> MAPKATLVKKFKGLAVGVGALLAAPPIMGLASYAVNGISSYLSITINSTTYDFAPLAQAVMVFGGIGLVAYG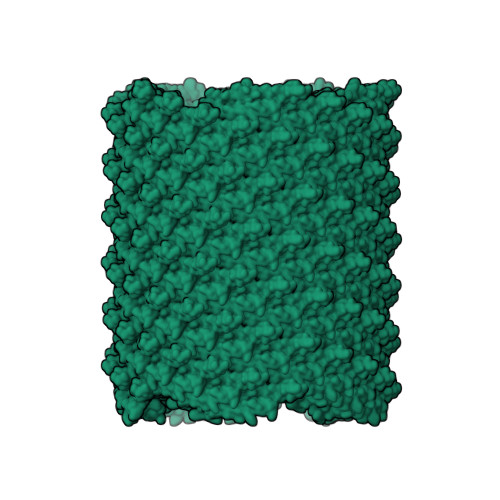LHRILGRGL>[6x]MK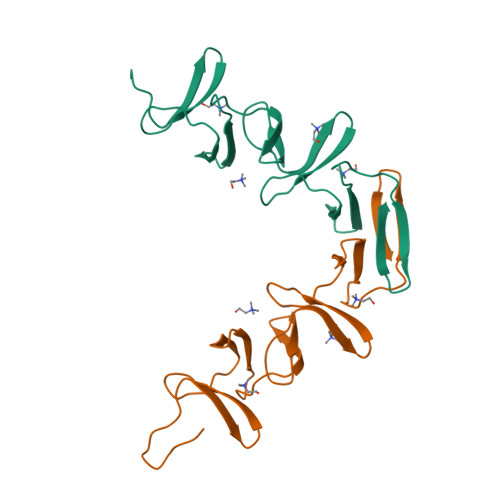GGIVHSDGSYPKDKFEKINGTWYYFDSSGYMLADRWRKHTDGNWYWFDNSGEMATGWKKIADKWYYFNEEGAMKTGWVKYKDTWYYLDAKEGAMVSNAFIQSADGTGWYYLKPDGTLADRPEFTVEPDGLITVK> MTPPLATTIDRLRDYLDRVGFQQIYKYIVAVNHYAVTPALITRNTAASVHHFFDSRLGGRAEFALLQCLMTGRPAEHAALPDKDRALADALVTAGLLRASPDGREVSGADRQLISAFGVDLLIDRRIHFGGEVHEVYIGPDSYWMLYYINASGIARTHRAVDLCTGSGIAALYLSLFTDHVLATDIGDVPLALVEINRRLNRRDAGTMEIRRENLNDTLD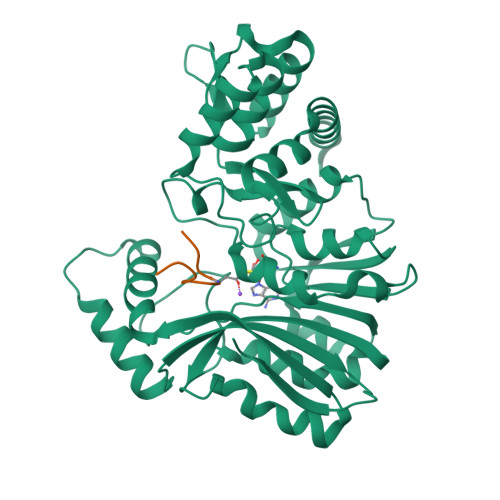GRERFDLLTCNPPFVAFPPGYSGTLYSQGTGVDGLGYMRDIVGRLPEVLNPGGSAYLVADLCGDAHGPHFLGELESMVTGHGMRIEAFIDHVLPASAQVGPISDFLRHAAGLPADTDIAADVQAFQRETLRADYYYLTTIRLQTAAQNPGLRMLRRDPLPGAGT;> AAAAVVTYLGAANVVGAANGTVTANAVANTNAVA>GSDSSRRQYQEKYKQVEQYMSFHKLPADFRQKIHDYYEHRYQGKMFDEDSILGELNGPLREEIVNFNCRKLVASMPLFANADPNFVTAMLTKLKFEVFQPGDYIIREGTIGKKMYFIQHGVVSVLTKGNKEMKLSDGSYFGEICLLTRGRRTASVRADTYCRLYSLSVDNFNEVLEEYPMMRRAFETVAIDRLDRDGKKN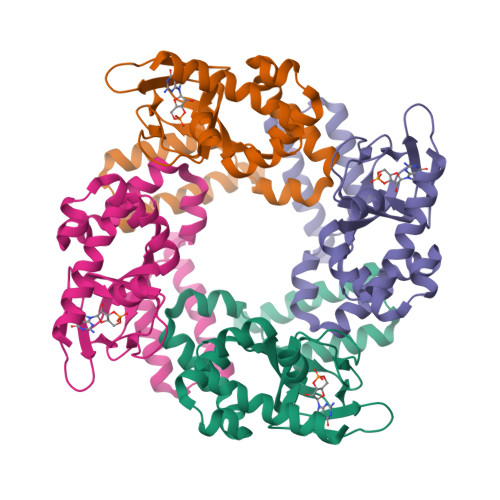[2x]> GSHMEYLGVFVDETKEYLQNLNDTLLELEKNPEDM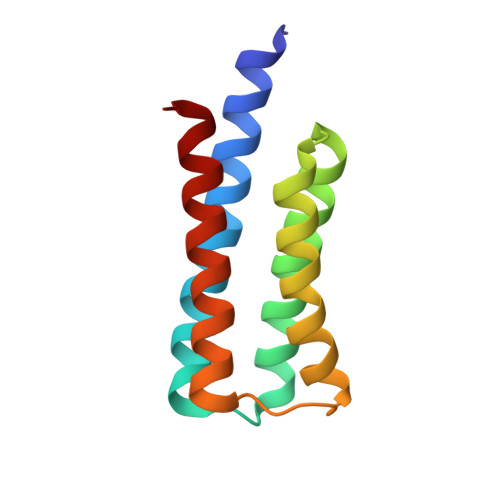ELINEAFRALHTLKGMAGTMGFSSMAKLCHTLENILDKARNSEIKITSDLLDKIFAGVDMITRMVDKIVS>RNGDLLLDHSGAYVAQYYITWNELSYDHQGKEVLTPKAWDRNGQDLTAHFTTSIPLKGNVRNLSV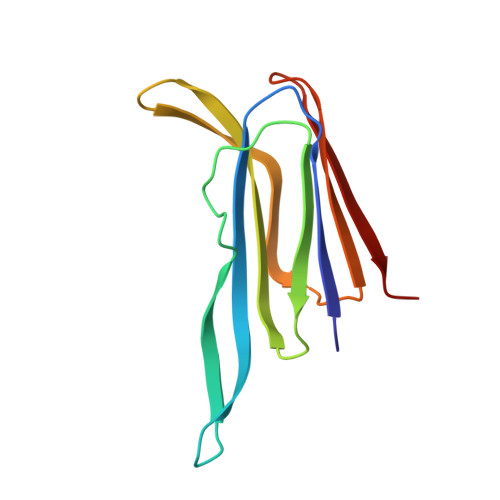KIRECTGLAWEWWRTVYEKTDLPLVRKRTISIWGTTLYPQVEDKVEND[2x]> GSQKERLLDELTLEGVARYMQSQRCRRVICLVGAGISTSAGIPDFRSPSTGLYDNLEKYHLPYPEAIFEISYFKKHPEPFFALAKEL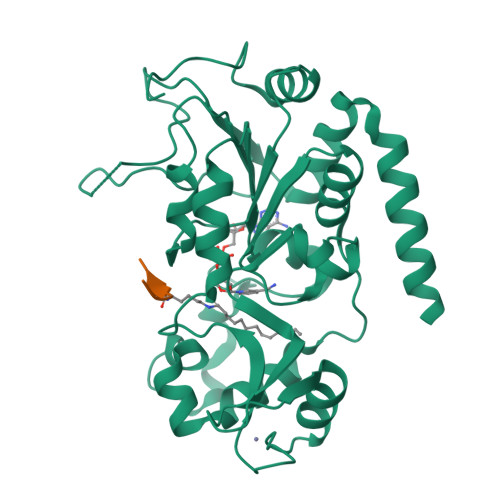YPGQFKPTICHYFMRLLKDKGLLLRCYTQNIDTLERIAGLEQEDLVEAHGTFYTSHCVSASCRHEYPLSWMKEKIFSEVTPKCEDCQSLVKPDIVFFGESLPARFFSCMQSDFLKVDLLLVMGTSLQVQPFASLISKAPLSTPRLLINKEKAGQSDPFLGMIMGLGGGMDFDSKKAYRDVAWLGECDQGCLALAELLGWKKELEDLVRREHASIDAQ;> PRKQLA>[2x]GGCCUAAAAGCAUAGUGGGAAAGUGACGUGAAAUUCGUCC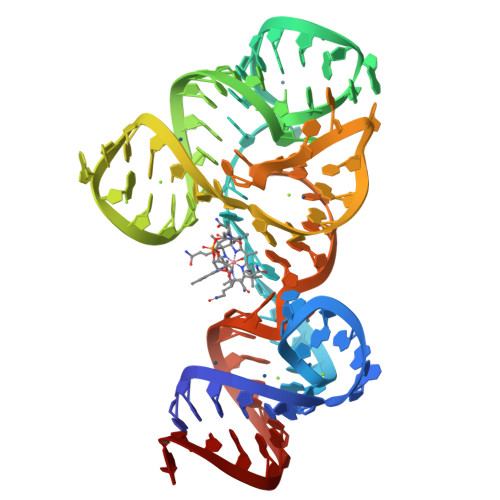AGAUGCGAAAGCAUACGGUUAUACUCCGAAUGCCACCUAGGCCA> MSQSNRELVVDFLSYKLSQKGYSWSQFSDVEENRTEAPEGTESEAVKQALREAGDEFELRYRRAFSDLTSQLHITPGTAYQSFEQVVNELFRDGVNWGRIVAFFSFGGALCVESVDKEMQVLVSRIAA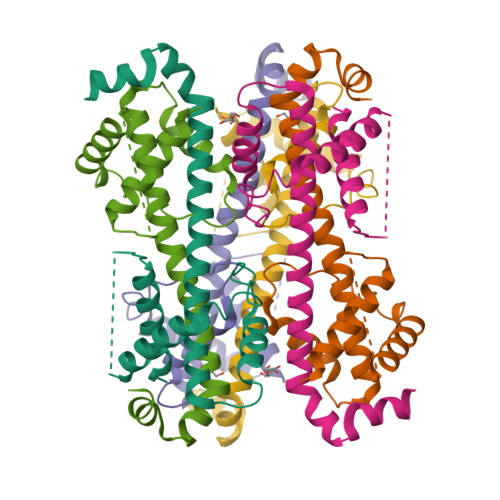WMATYLNDHLEPWIQENGGWDTFVELYGNNAAAESRKGQER>[4x]ACMRTYITNLNGHSITSTAQIAQNMVTDIAVSLGFRELGIHSYPIDTDSPEEMSKRLDGI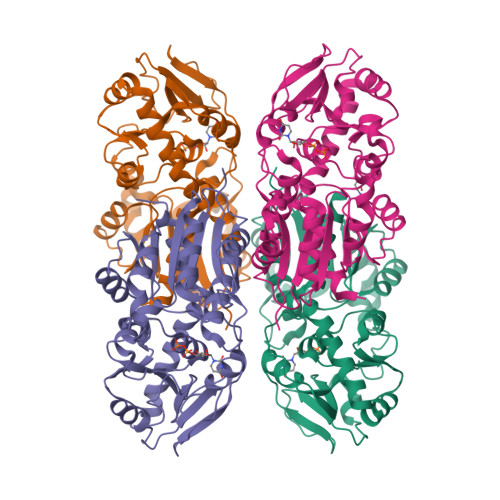CSGLRKNDIVIFQTPTWNTTTFDEKLFHKLKIFGVKIVIFIHDVVPLMFDGNFYLMDRTIAYYNEADVLIAPSQAMVDKLQSYGLTVKKILVQGMWDHPTNITLQAVNHKKLVHFPGNPERFNFIKNWRIPTELHVYTDHNMQLPTTVVKEPYQSDEQLIMKMSEGGYGLVWMDDRDKQYQSLYCPYKLGAYIAAGIPVIIQKGIANQDIIEKNNLGFIIEKIDDISNIVESTTEEEYMEIVSDVRRFNPLVRQGYFTRKLLTDAVFSALNSM>MASTKAPGPGEKHHSIDAQLRQLVPGKVSEDDKLIEYDALLVDRFLNILQDLHGPSLREFVQECYEVSADYEGKGDTTKLGELGAKLTGLAPADAILVASSILHMLNLANLAEEVQIAHRRRNSKLKKGGFADEGSATTESDIEETLKRLVSEVGKSPEEVFEALKNQTVDLVFTAHPTQSARRSLLQKNARIRNCLTQLNAKDITDDDKQELDEALQREIQAAFRTDEIRRAQPTPQDEMRYGMSYIHETVWKGVPKFLRRVDTALKNIGINERLPYNVSLIRFSSWMGGDRDGNPRVTPEVTRDVCLLARMMAANLYIDQIEELMFELSMWRCNDELRVRAEELHSSSGSKVTKYYIEFWKQIPPNEPYRVILGHVRDKLYNTRERARHLLASGVSEISAESSFTSIEEFLEPLELCYKSLCDCGDKAIADGSLLDLLRQVFTFGLSLVKLDIRQESERHTDVIDAITTHLGIGSYREWSEDKRQEWLLSELRGKRPLLPPDLPQTEEIADVIGAFHVLAELPPDSFGPYIISMATAPSDVLAVELLQRECGVRQPLPVVPLFERLADLQSAPASVERLFSVDWYMDRIKGKQQVMVGYSDSGKDAGRLSAAWQLYRAQEEMAQVAKRYGVKLTLFHGRGGTVGRGGGPTHLAILSQPPDTINGSIRVTVQGEVIEFCFGEEHLCFQTLQRFTAATLEHGMHPPVSPKPEWRKLMDEMAVVATEEYRSVVVKEARFVEYFRSATPETEYGRMN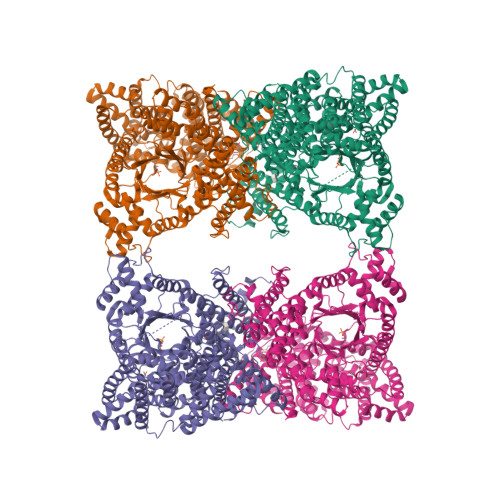IGSRPAKRRPGGGITTLRAIPWIFSWTQTRFHLPVWLGVGAAFKFAIDKDVRNFQVLKEMYNEWPFFRVTLDLLEMVFAKGDPGIAGLYDELLVAEELKPFGKQLRDKYVETQQLLLQIAGHKDILEGDPFLKQGLVLRNPYITTLNVFQAYTLKRIRDPNFKVTPQPPLSKEFADENKPAGLVKLNPASEYPPGLEDTLILTMKGIAAGMQNTG[2x]>MTPMKTYDLIVIGTGPGGYHAAIRAAQLGLKVLAVEAGEVGGVCLNVGCIPTKALLHAAETLHHLKVAEGFGLKAKPELDLKKLGGWRDQV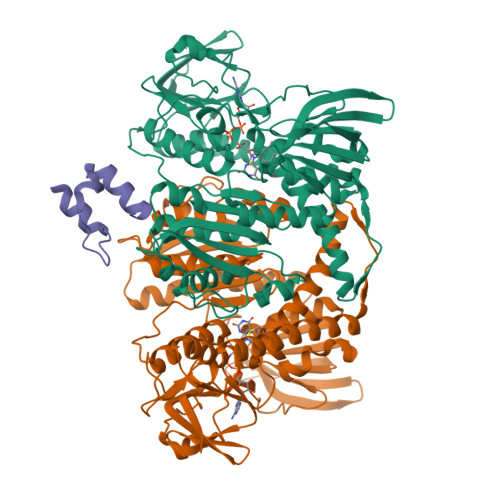VKKLTGGVGTLLKGNGVELLRGFARLVGPKEVEVGGERYGAKSLILATGSEPLELKGFPFGEDVWDSTRALKVEEGLPKRLLVIGGGAVGLELGQVYRRLGAEVTLIEYMPEILPQGDPETAALLRRALEKEGIRVRTKTKAVGYEKKKDGLHVRLEPAEGGEGEEVVVDKVLVAVGRKPRTEGLGLEKAGVKVDERGFIRVNARMETSVPGVYAIGDAARPPLLAHKAMREGLIAAENAAGKDSAFDYQVPSVVYTSPEWAGVGLTEEEAKRAGYKVKVGKFPLAASGRALTLGGAEGMVKVVGDEETDLLLGVFIVGPQAGELIAEAALALEMGATLTDLALTVHPHPTLSESLMEAAEAFHKQAIHILNR[4x];>PAAPSIRRLARELGVDLTRLRGTGLAGRITEEDVRRAAGL[2x]>[2x]MALDKLDLYVIITLVVAVAAYFAKNQFLDQPQDTGFLNTDSGSNSRDVLSTLKKNNKNTLLLFGSQTGTAEDYANKLSRELHSRFGLKTMVADFADYDWDNFGDITEDILVFFIVATYGEGEPTDNADEFHTWLTEEADTLSTLRYTVFGLGNSTYEFFNAIGRKFDRLLSEKGGDRFAEYAEGDDGTGTLDEDFMAWKDNVFDALKNDLNFEEKELKYEPNVKL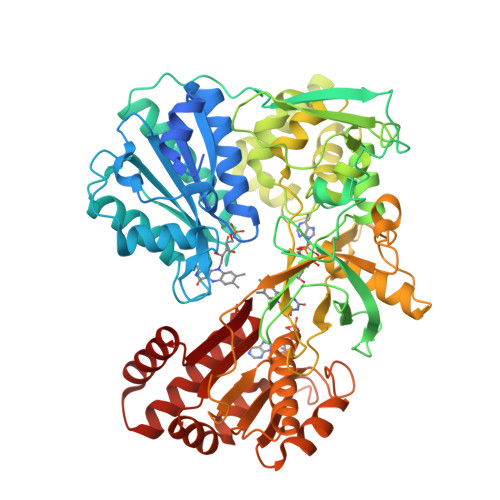TERDDLSAADSQVSLGEPNKKYINSEGIDLTKGPFDHTHPYLARITETRELFSSKERHCIHVEFDISESNLKYTTGDHLAIWPSNSDENIKQFAKCFGLEDKLDTVIELKALDSTYTIPFPTPITYGAVIRHHLEISGPVSRQFFLSIAGFAPDEETKKTFTRLGGDKQEFATKVTRRKFNIADALLYSSNNTPWSDVPFEFLIENIQHLTPRYYSISSSSLSEKQLINVTAVVEAEEEADGRPVTGVVTNLLKNIEIAQNKTGEKPLVHYDLSGPRGKFNKFKLPVHVRRSNFKLPKNSTTPVILIGPGTGVAPLRGFVRERVQQVKNGVNVGKTLLFYGCRNSNEDFLYKQEWAEYASVLGENFEMFNAFSRQDPSKKVYVQDKILENSQLVHELLTEGAIIYVCGDASRMARDVQTTISKIVAKSREISEDKAAELVKSWKVQNRYQEDVW> AMNTDLKLPAGKTMTIEDVKQLLERY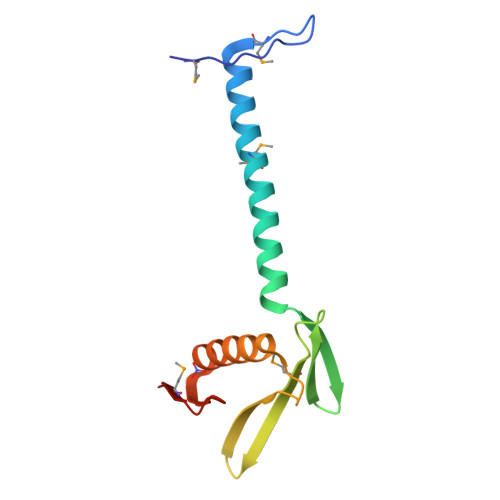QMALKKTGEQLGWAYEQAAFPYTVRIHESVLYLQGDGRLYKGMAISVRTAGEETFIDIALPPGATHGDKGKANEFSKWLAKTLGGELHLFSGRTMVFGSA[4-[5-(7-fluoranylquinolin-4-yl)-1-methyl-imidazol-4-yl]-3,5-dimethyl-phenyl]methanamine | C22 H21 F N4 | 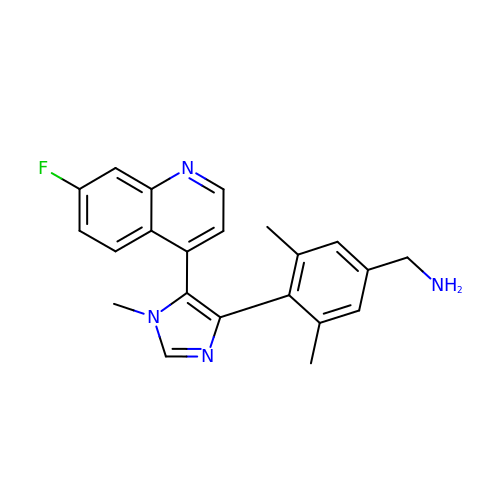WOAOENGFAAUUGT-UHFFFAOYSA-N> LQF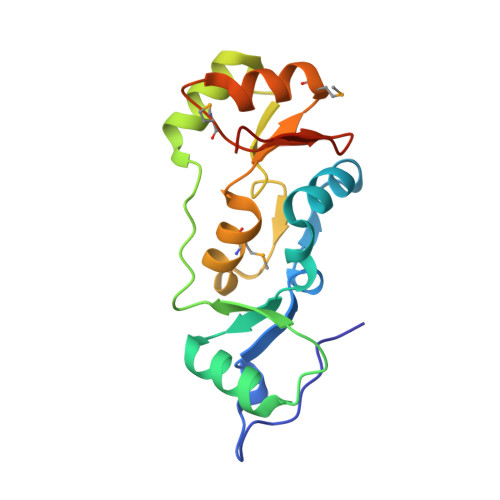AYKDPEKNWNRNSVKGLVASLINVKDNSTATALEVVAGERLYNVVVDTEVTAKKLLEKGELKRRYTIIPLNKISARCIAPETLRVAQNLVGPDNVHVALSLVDYKPELQKGMEFVFGTTFVCNNMDNAKKVAFDKRIMTRTVTLGGDVFDPHGTLSGG>GPGSSLSRFRGCLAGALLGDCVGSFYAAHDTVDLTSVLRHVQSLEPDPGTPGSERTEALYYTDDTAMARALVQSLLAKEAFDEVDMAHRFAQEYKKDPDRGYGAGVVTVFKKLLNPKCRDVFEPARAQFNGKGSYGNGGAMRVAGISLAYSSVQDVQKFARLSAQLTHASSLGYNGAILQALAVHLALQGESSSEHFLKQLLGHMEDLEGDAQSVLDARELGMEERPYSSRLKKIGELLDQASVTREEVVSELGNGIAAFESVPTAIYCFLRCMEPDPEIPSAFNSLQRTLIYSISLGGDTDTIATMAGAIAGAYYGMDQVPESWQQSCEGYEETDILAQSLHRVFQKS[4x];>PAKSAPAPKKG[4x]

Poly(ADP-ribose)glycohydrolase (PARG) and (ADP-ribosyl)hydrolase 3 (ARH3) are the main hydrolases of serine PAR- and MARylation, respectively, thus playing a pivotal role in signal silencing following DNA damage. ARH3 is the only known enzyme to reverse serine MARylation and is consequently responsible for the regulation of hundreds of ADP-ribosylated proteins following DNA damage. In contrast to PARG, the active site of ARH3 contains a catalytic binuclear magnesium centre. To understand the impact of the ARH3:substrate interaction on reaction efficiency, we crystallised ARH3 in complex with the chemically synthesised substrates: histone H2B peptide (aa 1–11) MARylated on Ser7 (H2BS7mar), dimeric ADP-ribose (dimer) and α-NAD+.

Therefore, we chose to crystallise the hARH3 E41A substrate complexes as this prevents substrate cleavage during crystal formation, while retaining a functionally relevant magnesium coordination. The H2BS7mar peptide lies loosely coordinated within a groove running perpendicularly to the ADPr binding cleft. It adopts no secondary structure and makes mostly water-mediated contacts with the hARH3 protein. This binding mode is incompatible with the closed conformation of the Glu41-flap and indeed stabilises the open form via a Lys6 (side chain, H2B peptide):Glu41(backbone, hARH3) contact, which is part of the short serine-ADP-ribosylation consensus motif (KS). H2BS7mar and meADPr act similarly to chelants via the 1″ and 2″ oxygens. In addition, the backbone-carbonyl of peptide Ser7 occupies the axial position of MgII. The interactions with either H2BS7mar or meADPr increase the Thr317-MgII distance by 0.9–1.6 Å relative to the ADPr-bound state, which breaks the coordinating bond and leads to an unusual five-coordinated distorted square-pyramidal geometry around the Mg2+ ion. In the hARH3:H2BS7mar complex, Glu41 is shielded from the aqueous environment by the peptide and is no longer able to form a first-order coordination bond with MgII. Noteworthy, neither the H2BS7mar nor the α-NAD+ complex have a water ligand at MgII, thus excluding the ion as a water activator during the reaction cycle.2-(hydroxymethyl)cyclopent-2-en-1-one | C6 H8 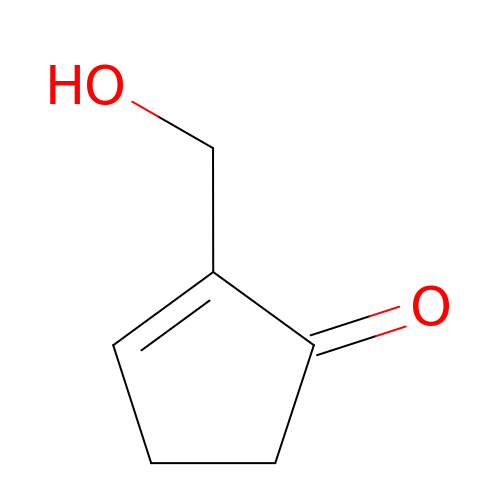O2 | DQTFESRTIZHRRO-UHFFFAOYSA-N> DLTVKEKEELIEEWQPEPLVPPVPKDHPALNYNIVSGPPSHKTVVNGKECINFASFNFLGLLDNPRVKAAALASLKKYGVGTCGPRGFYGTFDVHLDLEDRLAKFMKTEEAIIYSYGFATIASAIPAYSKRGDIVFVDRAACFAIQKGLQASRSDIKLFKHNDMADLERLLKEQEIEDQKNPRKARVTRRFIVVEGLYMNTGTICPLPELVKLKYKYKARIFLEESLSFGVLGEHGRGVTEHYGINIDDIDLISANMENALASIGGFCCGRSFVIDHQRLSGQGYCFSASLPPLLAAAAIEALNIMEENPGIFAVLKEKCGQIHKALQGISGLKVVGESLSPAFHLQLEESTGSREQDVRLLQEIVDQCMNRSIALTQARYLEKEEKCLPPPSIRVVVTVEQTEEELERAASTIKEVAQAVLL;> MRPEPGGCCCRRTVRANGCVANGEVRNGYVRSSAAAAAAAAAGQIHHVTQNGGLYKRPFNEAFEETPMLVAVLTYVGYGVLTLFGYLRDFLRYWRIEKCHHATEREEQKDFVSLYQDFENFYTRNLYMRIRDNWNRPICSVPGARVDIMERQSHDYNWSFKYTGNIIKGVINMGSYNYLGFARNTGSCQEAAAKVLEEYGAGVCSTRQEIGNLDKHEELEELVARFLGVEAAMAYGMGFATNSMNIPALVGKGCLILSDELNHASLVLGARLSGATIRIFKHNNMQSLEKLLKDAIVYGQPRTRRPWKKILILVEGIYSMEGSIVRLPEVIALKKKYKAYLYLDEAHSIGALGPTGRGVVEYFGLDPEDVDVMMGTFTKSFGASGGYIGGKKELIDYLRTHSHSAVYATSLSPPVVEQIITSMKCIMGQDGTSLGKECVQQLAENTRYFRRRLKEMGFIIYGNEDSPVVPLMLYMPAKIGAFGREMLKRNIGVVVVGFPATPIIESRARFCLSAAHTKEILDTALKEIDEVGDLLQLKYSRHRLVPLLDRPFDETTYEETED;> MADYKDDDDKSGPDEVDASGRMAGMALARAWKQMSWFYYQYLLVTALYMLEPWERTVFNSMLVSIVGMALYTGYVFMPQHIMAILHYFEIVQ;> MNVGTAHSEVNPNTRVMNSRGIWLSYVLAIGLLHIVLLSIPFVSVPVVWTLTNLIHNMGMYIFLHTVKGTPFETPDQGKARLLTHWEQMDYGVQFTASRKFLTITPIVLYFLTSFYTKYDQIHFVLNTVSLMSVLIPKLPQLHGVRIFGINKY;> MATATEQWVLVEMVQALYEAPAYHLILEGILILWIIRLLFSKTYKLQERS

The ORM/ORMDL family proteins function as regulatory subunits of the serine palmitoyltransferase (SPT) complex, which is the initiating and rate-limiting enzyme in sphingolipid biosynthesis. In humans, the heterotrimeric SPT core enzymatic complex, composed of SPTLC1, SPTLC2 or SPTLC3, and SPTssa or SPTssb, catalyzes the first and rate-limiting step of de novo sphingolipid biosynthesis by condensation of serine and palmitoyl-CoA to generate 3-keto-dihydrosphingosine (3-KDS). As a critical mechanism for the homeostatic regulation of sphingolipid production, SPT activity is inhibited in response to elevated cellular sphingolipid levels in an ORM/ORMDL-dependent manner. In this work, we demonstrate that ceramide binds directly with and inhibits the human SPT-ORMDL complexes, a process that is important for establishing cellular sphingolipid homeostasis.

To investigate the structural basis for SPT-ORMDL regulation by ceramide, we determined the structure of the SPT-ORMDL3 complex in the presence of excess C6-ceramide using single-particle cryo-EM. The structure of the monomeric SPT-ORMDL3 complex was resolved at an overall resolution of 2.9 Å. Compared to the cryo-EM map of the monomeric SPT-ORMDL3* complex we previously reported, several extra well-ordered lipid-like densities could be resolved between ORMDL3 and SPTLC2 in the cytosolic membrane leaflet. While the N-terminus of ORMDL3* was not resolved in the SPT-ORMDL3* structure, the N-terminus of ORMDL3 could be well resolved in the updated maps. Among the well-ordered lipid-like densities, the shape and size of one lipid-like density are consistent with a C6-ceramide molecule, showing one small polar head contiguous with two acyl chains. Close to the C6-ceramide density, we could observe two additional lipid-like densities, which might result from the acyl chains of phospholipids, sphingolipids, or other lipidic species. An alternative explanation for the two presumable acyl-chain densities is that they might arise from the average of C6-ceramide and endogenous bound long-chain ceramide (such as C24-ceramide). In the ceramide binding site, the polar head of ceramide makes five potential hydrogen bonds with the surrounding residues, including the side chain groups of Asn13 and His85 in ORMDL3, Tyr122 in SPTLC2, and the main chain group of Phe63 in ORMDL3 (left). The two aliphatic chains of ceramide are enclosed by numerous hydrophobic residues from both ORMDL3 and SPTLC2.A well‐studied, DNA tensegrity triangle crystal were explored as a crystal scaffold to regularly arrange DNA T‐junction motifs in 3D space. T‐junction is a T‐shaped, structural motif designed by Satoshi Murata and Hamada Shogo. It is formed by hybridization between a single‐stranded DNA (ssDNA) sticky end (black) of a DNA duplex and a ssDNA bulge loop of another DNA duplex (green). For structural characterization, a T‐junction is incorporated at the center helical domain of each component duplex of the triangle, resulting in a modified, T‐junction triangle (ΔT) motif. The T‐junction triangle is named as ΔTm‐n. ΔT stands for T‐junction‐containing triangle; numbers m and n indicate the distance (in base pairs, bps) between the hairpin and the left corner of the triangle and the length (in bps) of the side duplex arm (C‐arm), respectively.

The crystals of all the ΔT variants were studied by X‐ray crystallography. They all shared R3 rhombohedral lattices with the same unit cell dimensions: a = b = c ∼100 Å and α = β = γ = 112 – 114°. The data matched with the parameters of conventional 3‐turn tensegrity triangle crystals within 3% error; indicating that the overall DNA triangle frameworks remained the same for all ΔT variants. Indeed, for all ΔT variants, extra densities (colored green) could clearly be identified (e for ΔT7‐6, S3d and S3e for ΔT6‐6, S4d and S4e for ΔT6‐11, S5d and S5e for ΔT7‐11, S6d and S6e for ΔT8‐6, S7d and S7e for ΔT8‐11). In ΔT6‐6 and ΔT6‐11, the extra densities were directly below the triangle planes. For crystals with the same C‐arm positions, the orientations and the locations of the extra C‐arms were almost identical. When the C‐arm position was the same, the triangles could pretty much completely overlap with each other, ΔT6‐6/ΔT6‐11, ΔT7‐6/ΔT7‐11, and ΔT8‐6/ΔT8‐11, except the C‐arm lengths. More interesting was superimposing the triangles with C‐arms of the same length but different C‐arm positions, ΔT6‐6/ΔT7‐6/ΔT8‐6/ and ΔT6‐11/ΔT7‐11/ΔT8‐11/. By looking along the triangle edge duplex, the C‐arms rotated stepwise by 28°–54° (rotating angles from ΔT6‐6 to ΔT7‐6 to ΔT8‐6 are 28° and 54°, respectively; rotating angles from ΔT6‐11 to ΔT7‐11 to ΔT8‐11 are 43° and 37°, respectively), consistent with the twist of 34°/bp for B‐DNA duplex.

> CAGCAGCCTGAATA;> GGCTGC;> GCGAGTATTCACCGGCTCCGCGGACAACTTTTGTTGTCCGCGGCTCGCAGCCGGACAGCG;> TGCGCTGT5-(4'-AMINO-1'-ETHYL-5',8'-DIFLUORO-1'H-SPIRO[PIPERIDINE-4,2'-QUINAZOLINE]-1-YLCARBONYL)PICOLINONITRILE | C21 H22 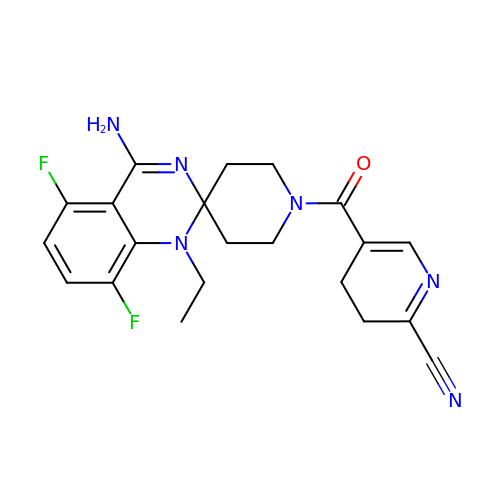F2 N6 O | QCFIRACCCDFXIP-UHFFFAOYSA-N> HDDFADD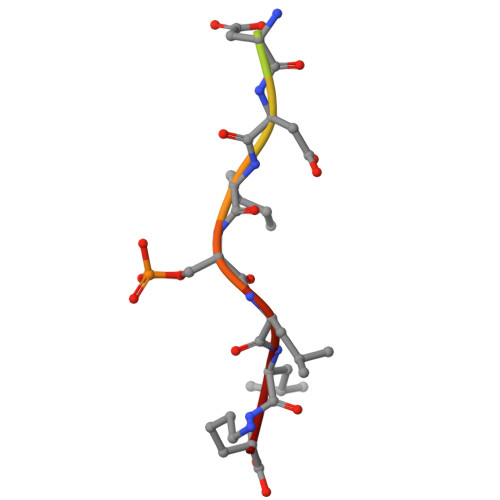ISLLK1-[2-HYDROXY-3-(4-CYCLOHEXYL-PHENOXY)-PROPYL]-4-(2-PYRIDYL)-PIPERAZINE | C24 H33 N3 O2 | 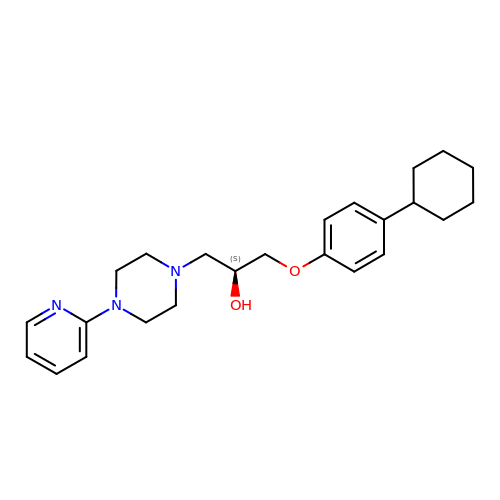BZJHCQBNFUNZPJ-QFIPXVFZSA-N>MQKRAIYPGTFDPITNGHIDIVTRATQMFDHVILAIAASPSKKPMFTLEERVALAQQATAHLGNVEVVGFSDLMANFARNQHATVLIRGLRAVADFEYEMQLAHMNRHLMPELESVFLMPSKEWSFI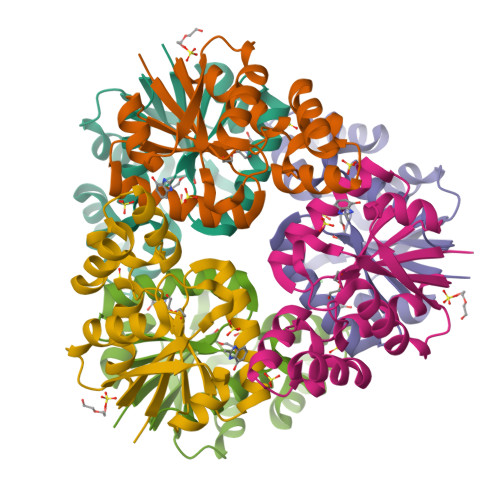SSSLVKEVARHQGDVTHFLPENVHQALMAKLAVDHHHHHH[2x]> VDECWRIIASHTWFCA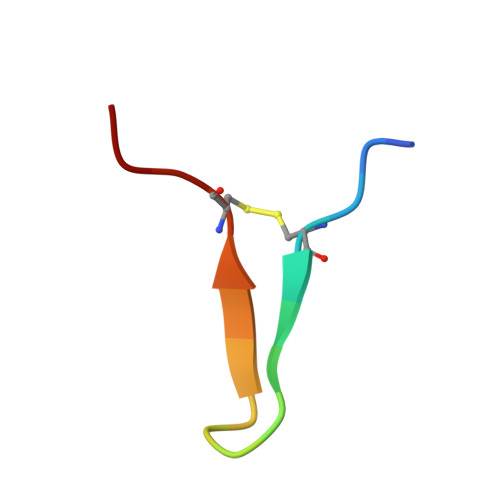EE5-BROMOQUINOLINE | C9 H6 Br N | 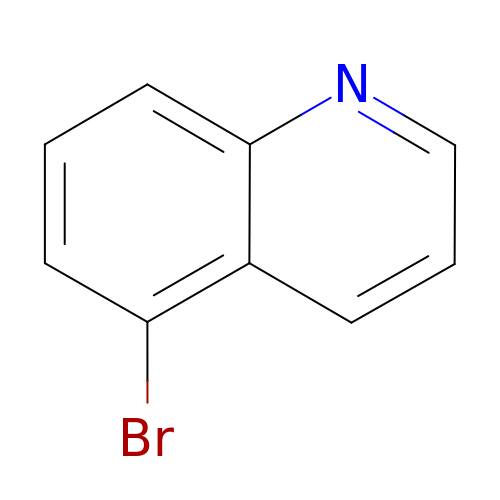CHODTZCXWXCALP-UHFFFAOYSA-N> AECSVDIQGNDQMQFNTNAITVDKSCKQFTVNLSHPGNLPKNVMGHNWVLSTAADMQ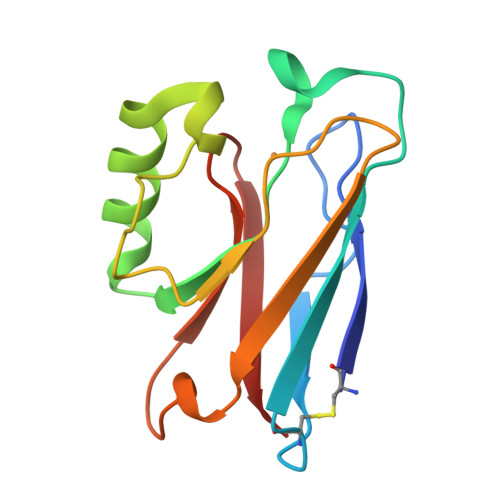GVVTDGMASGLDKDYLKPDDSRVIAHTKLIGSGEKDSVTFDVSKLKEGEQYMFFCTPHPMKGTLTLK>[2x]MR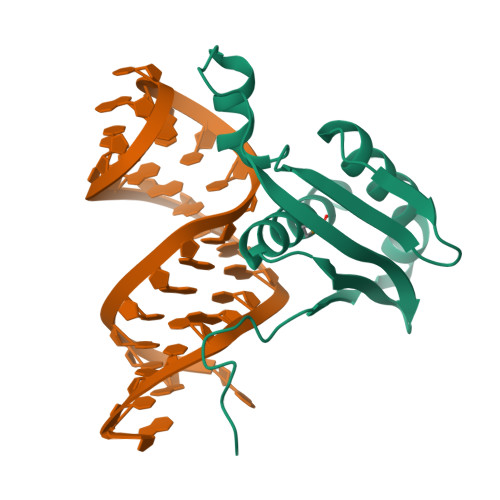PHNELIRPSSTSLSKYFPHKVLQNWTLDPELCAQIDDILQKFLDDNKIPWSKKGSVLEISTKSITWSRKARRISKSQTSVSSLEGQMKCELNVIDNQLQCKWIEGYDYNVYESFCSALARALRDNKK> KETAAAKFERQAMDSSTSAASSSNYCNQMMKSRNLTKDRCKP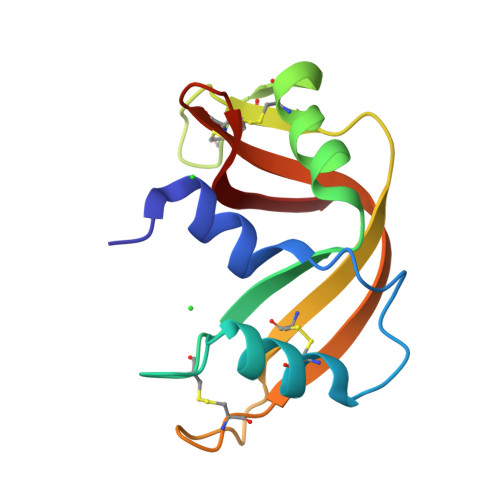VNTFVHESLADVQAVCSQKNVACKNGQTNCYQSYSTMSITDCRETGSSKYPNCAYKTTQANKHIIVACEGNPYVPVHFDASV1-MENAPHTHYL GLUTATHIONE 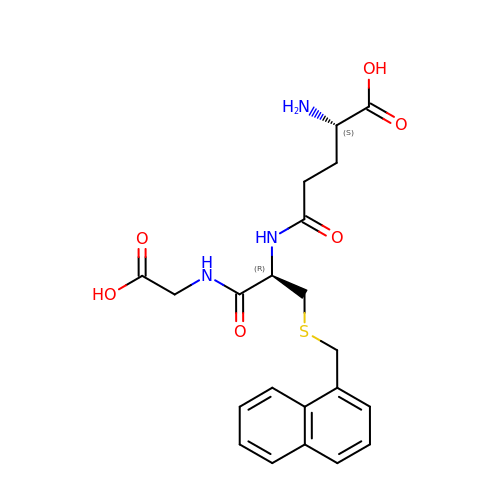CONJUGATE | C21 H25 N3 O6 S | IHZCIRSQSFPOLH-IRXDYDNUSA-N>[8x]GIIEFHVIGNSLTPKANRRVLLWLVGLQNVFSHQLPRMPKEYIARLVFDPKHKTLALIKDGR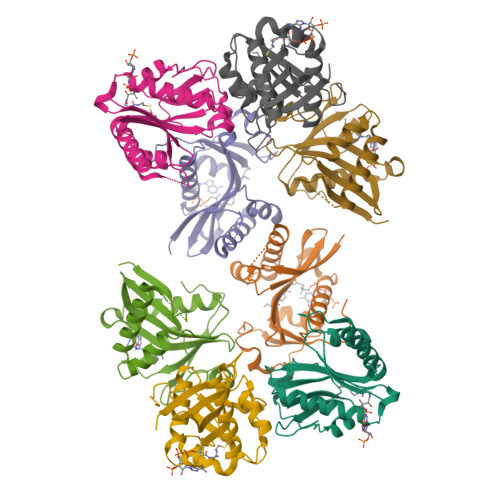VIGGICFRMFPTQGFTEIVFCAVTSNEQVKGYGTHLMNHLKEYHIKHNILYFLTYADEYAIGYFKKQGFSKDIKVPKSRYLGYIKDYEGATLMECELNPRIPYT>LAPPYRVILHNDNFNKRE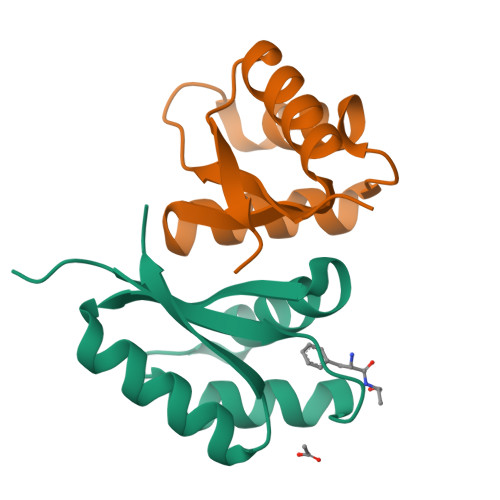YVVQVLMKVIPGMTVDNAVNIMQEAHINGLAVVIVCAQADAEQHCMQLRGNGLLSSVEPDGGGC[2x]> GEFTQSVSRLQSIVAGLKNAPSDQLINIFESCVRNPVENIMKILKGIGETFCQHYTQSTDEQPGSHIDFAVNRLKLAEILYYKILETVMVQETRRLHGMDMSVLLEQDIFHRSLMACCLEIVL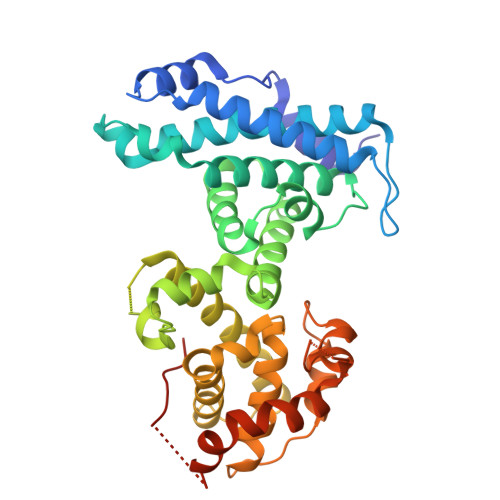FAYSSPRTFPWIIEVLNLQPFYFYKVIEVVIRSEEGLSRDMVKHLNSIEEQILESLAWSHDSALWEALQVSANKVPTCEEVIFPNNFETGRPKRTGSLALFYRKVYHLASVRLRDLCLKLDVSNELRRKIWTCFEFTLVHCPDLMKDRHLDQLLLCAFYIMAKVTKEERTFQEIMKSYRNQPQANSHVYRSVLLKSIKEERGDLIKFYNTIYVGRVKSFALKYDLANQDHMMDAPPLSPFPHIKQQ Glutaminyl-peptide cyclotransferases (QCs) convert the N-terminal glutamine or glutamate residues of protein and peptide substrates into pyroglutamate (pE) by releasing ammonia or a water molecule. The N-terminal pE modification protects peptides/proteins against proteolytic degradation by amino- or exopeptidases, increasing their stability. Indeed, its crystal structure revealed that a Zn(II) ion bound in a tetrahedral coordination to Asp159, Glu202, His330, and to a water molecule. All X-ray crystallography experiments were performed using the hQC double mutant Y115E-Y117E (hQC-2X), formerly validated by us as a soluble protein variant exploitable for drug discovery purposes.

The crystal structure of apo-hQC-2X was determined to be 1.96 Å resolution, in the monoclinic space group C2. The crystal asymmetric unit (ASU) contains three independent molecules that are almost identical within experimental errors (pairwise root-mean-square deviation, RMSD, values of 0.11–0.14 Å). The tertiary structure of hQC-2X, having the mixed α/β hydrolase fold with an open sandwich topology, is not affected by the removal of the functional metal cofactor. Indeed, the structural comparison between apo-hQC-2X and the holo-enzyme shows no meaningful difference, as indicated by RMDS values ranging from 0.21 Å to 0.24 Å. This evidence suggests that the binding of the metal cofactor, although critical for the catalytic function, is not necessary for the enzyme to acquire the proper folding. Upon removal of the metal ion, a water molecule, WatC, populates the cofactor binding pocket in all three subunits composing the ASU. WatC donates two H-bonds to Asp159 and Glu202 and receives from His330 and a further water molecule (Wat2), placed inside the catalytic cavity and bound to Trp329. On the opposite wall, the indole moiety of Trp207 is rotated inside the catalytic cavity, contributing to the cone-shaped active site. The crystal structure of apo-hQC underlines the robustness of the hQC active site cavity that maintains its structure even without the metal ion. On the other hand, this scarcely flexible cavity indicates quite strict requirements for molecules that can be hosted as either substrates or inhibitors.

>MRGSHHHHHHGSASAWPEEKNYHQPAILNSSALRQIAEGTSISEMWQNDLQPLLIERYPGSPGSYAARQHIMQRIQRLQADWVLEIDTFLSQTPEGERSFSNIISTLNPTAKRHLVLACHYDSKYFSHWNNRVFVGATDSAVPCAMMLELARALDKKLLSLKTVSDSKPDLSLQLIFFDGEEAFLHWSPQDSLYGSRHLAAKMASTPHPPGARGTSQLHGMDLLVLLDLIGAPNPTFPNFFPNSARWFERLQAIEHELHELGLLKDHSLEGRYFQNYSYGGVIQDDHIPFLRRGVPVLHLIPSPFPEVWHTMDDNEENLDESTIDNLNKILQVFVLEYLHL[3x]(2S)-1-(4,4-dimethylpiperidin-1-yl)-3-{3-[3-({[(4-fluorophenyl)methyl]amino}methyl)-4-(trifluoromethyl)phenyl]-5-(methylsulfonyl)-4,5,6,7-tetrahydro-1H-pyrazolo[4,3-c]pyridin-1-yl}propan-2-ol 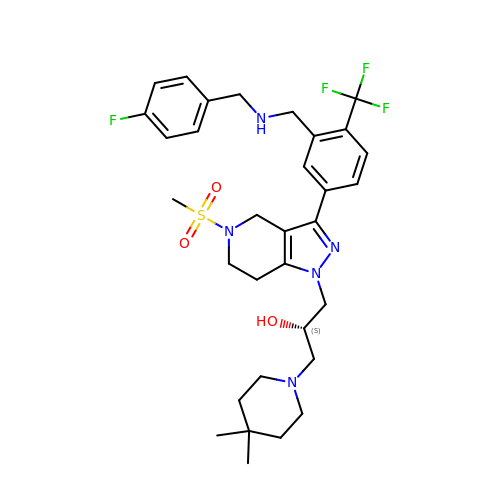| C32 H41 F4 N5 O3 S | QCRLHLMORQICFX-SANMLTNESA-N> GHIKQLLKNKRFEVIKALVESKKIKQEWLEDLYSILLKQDTDVEITQAKYEIIKLLLTEKKYLNFELLTKTLNLDQQTAIEIMRNPFKEVYFPTYNIENPEESRLNKALIIPLSNQTFTLNTFVNSQDLETIKEATNKNFFVIFDNIFSGKSYQLAVAAGLIAKEKEILDNVAFTGEVSSNGFIIPVNHLEEKKEITEKAKKVLITPEDIENLEELSFWLNPEHLPVIFIHINKPELALQSLKQMEDAIKKDERFKYFKLENLKKFYRLEDQDMYLITPSVDFSNREELIKILNEFREKVSKLLTLEGVIK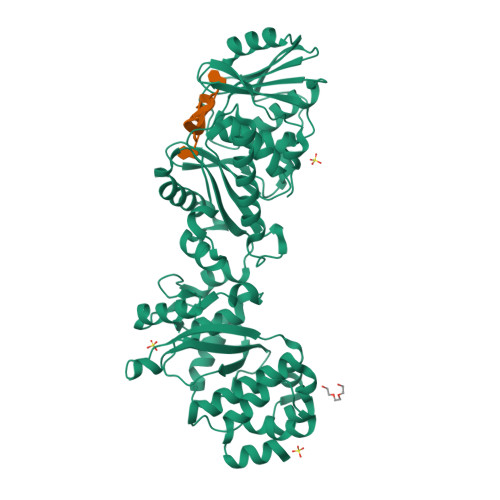DHNKVVLNISAGISTLALYFGVILGNRQASIIYHYQKEYHKVIDLTDNPRKIKEKKSEFEKISVNKNIQDPLMIIIYLASHNPIEKGLELKEKLRAKGELIIQSKEHQGNLEIGDWSDIVSEIYTAIDDNKQKENYMVFSAPVAIMLALGMALGYFLPIKVFHYNRDEYIEVPIKLNEEILRSPFPGE>PLTDTDRSEDFLRRVRGLKAARTANGPRLYQPITLLWAVGRARRGEARTLAWADTDEAIGALLKRHGARGERPRPDYPVLALHRAGLWTLEGHVGEVPTAHGDSALRNWFAEQRPVGGLAEPFHDLLHRSGHSRVSVIEALLTTYFAGLDPVPLLEDTGLYDEGHHHHH[2x]

The sulfur atom of phosphorothioated DNA (PT-DNA) is coordinated by a surface cavity in the conserved sulfur-binding domain (SBD) of type IV restriction enzymes. The sulfur modification-dependent REases SprMcrA and ScoMcrA use an SBD to recognize the DNA backbone phosphorothioate link of the RP stereoisomer, which is adopted by the naturally occurring PT modifications in five DNA core sequence contexts in prokaryotes. By contrast, the SBD of the PT-dependent restriction endonuclease (REase) SprMcrA from Streptomyces pristinaespiralis has a relatively relaxed sequence specificity, targeting GPSGCC, GPSAAC and GPSATC, but not GPSTTC or CPSCA. The sulfur atom of the PT linkage was inserted into a cavity which formed by Y31, Q32, Y78, P79 and A82 through Van der Waals interactions; the phosphate groups flanking the PT linkage formed electrostatic bonds with R29, R73 and R85, as well as hydrogen bonds with Y31 and A101.

Crystals for SBDSpr in complex with the RP form of the 10-bp hemi-PT DNA oligonucleotide 5′-GGCGPSAACGTG-3′ were grown and obtained at 14°C with the reservoir solution containing 0.1 M BIS-Tris pH 5.5, 0.15 M ammonium acetate, and 25% PEG 3350. The structure of the SBDSpr-GPSAAC complex was refined and rebuilt using Coot and Phenix.refine. SBDSpr showed the highest binding affinity for GPSGCC, with a dissociation constant value (KD) of 5.55 nM, followed by a KD of 38.33 nM for GPSATC and 94.67 nM for GPSAAC. It's worth noting that the ND1 atom of H102 also formed H-bond with N7 atom of G4 in GPSGCC and GPSAAC sequences, while this H-bond was not existing in SBDSpr-GPSATC complex. The N atom in the main chain of G103 bonded to N7 atom of SG5 from GPSGCC sequence and N7 atom of SA5 from GPSATC and GPSAAC sequences. In conclusion, HGD motif formed five H-bonds in SBDSpr–GPSGCC complex while four H-bonds in SBDSpr–GPSATC and SBDSpr–GPSAAC complexes, which explained why SBDSpr showed a highest affinity for GPSGCC. The base recognition pattern by HGD motif in complexes of SBDSpr–GPSAAC and SBDSpr–GPSATC is different. What's more, close comparison of two structures revealed that the binding of the GPSAAC released the methyl group of T6′ on the complementary strand from the binding site, and converts the weak non-bonded interaction to unfavored thymine methyl-solvent accessibility. In the case of GPSAAC, the T6′ methyl group was fully exposed to solvent and lack of specific interaction with SBD protein. Difference in the weak non-bonded interaction between GPSATC and GPSAAC results in a lower KD values for GPSATC than GPSAAC bound by SBDSpr.>GSAMDSSRRQYQEKYKQVEQYMSFHKLPADFRQKIHDYYEHRYQGKMFDEDSILGELNGPLREKIVNFNCRKLVASMPLFANADPNFVTAMLTKLKFEVFQPGDYIIREGTIGKKMYFIQHGVVSVLTKGNKEMKLSDGSYFGEICLLTRGRRTASVRADTYCRLYSLSVDNFNEVLEEYPMMRRAFETVAIDRLDRIGKKN[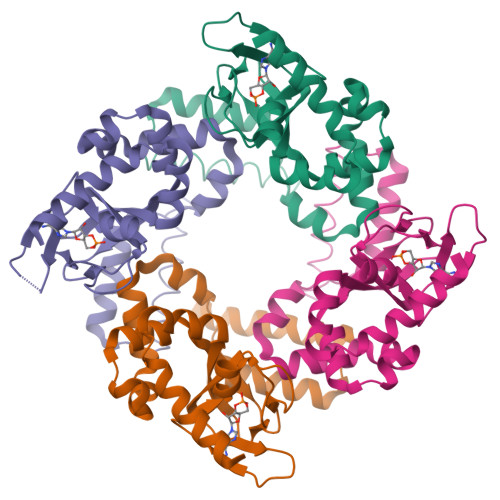4x]> APKAPADGLKMDKTKQPVVFNHSTHKAVKCGDCHHPVNGKENYQKCATAGCHDNMDKKDKSAKGYYHAMHDKGTKFKSCVGCHLETAGADAAKK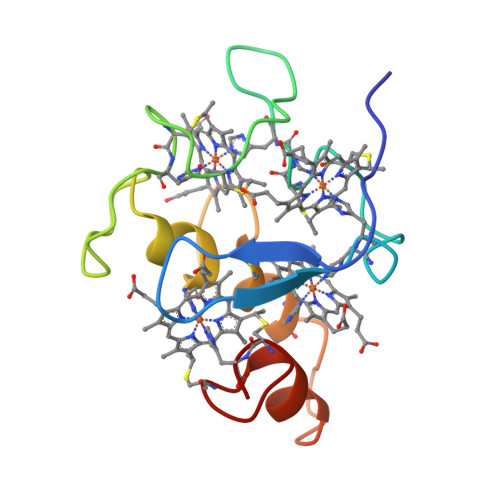KELTGCKGSKCHS The gp43 DNA polymerase of the RB69 bacteriophage (RB69 Pol) bears primary responsibility for the faithful and efficient replication of the viral genome. RB69 Pol belongs to the B-class of DNA polymerases and is closely related to T4 phage DNA polymerase. RB69 DNA Pol synthetizes DNA with high accuracy, introducing one mutation per 2 x 108 replicated bases. This high fidelity is achieved through the combined action of its polymerase (Pol) and 3′-5′-exonuclease (Exo) activities, which enable stringent selection of the correct incoming nucleotide and excision of the mismatches resulting from misincorporations.

Therefore, we took advantage of the Y567A substitution that has been shown to improve crystal quality without affecting the catalytic parameters of the enzyme (and references therein). We obtained crystals of a complex of the mutant polymerase, DNA and the dGpnpp non-hydrolyzable analog that diffracted to 2.30 Å resolution (ternary complex I). As expected, the ternary complex structure reveals an assembled active site with dGpnpp occupying the incoming dNTP binding pocket. Strikingly, however, while the base and sugar of the incoming nucleotide are found in positions that are consistent with other RB69 polymerase structures, both molecules in the ASU present an altered conformation for the three phosphate groups. As a consequence the α-phosphate is not properly aligned for catalysis. Furthermore, the D714A substitution drastically affects the metal coordination. Neither the dNTP binding metal, nor the catalytic metal ions are found in their expected positions. Interestingly, this aberrant active site conformation correlates with similar changes to those observed in the apo crystal structure, suggesting that the altered position of the incoming nucleotide is related to the conformation of D411 and, in turn, to the missing D714 side chain. As seen in the apo mutant structure, the D411 is flipped away from the active site and this correlates with the repositioning of the E686 and E716 side chains. Thus, the absence of the D714 side chain seems to cause the movement of the key metal-ligating D411 residue in the polymerase pocket and, as such, agrees with the observed decrease in the DNA polymerization rate.

>[2x]MKEFYLTVEQIGDSIFERYIDSNGRERTREVEYKPSLFAHCPESQATKYFDIYGKPCTRKLFANMRDASQWIKRMEDIGLEALGMDDFKLAYLSDTYNYEIKYDHTKIRVANFDIEVTSPDGFPEPSQAKHPIDAITHYDSIDDRFYVFDLLNSPYGNVEEWSIEIAAKLQEQGGDEVPSEIIDKIIYMPFDNEKELLMEYLNFWQQKTPVILTGWNVESFAIPYVYNRIKNIFGESTAKRLSPHRKTRVKVIENMYGSREIITLFGISVLDYIDLYKKFSFTNQPSYSLDYISEFELNVGKLKYDGPISKLRESNHQRYISYNIIAVYRVLQIDAKRQFINLSLDMGYYAKIQIQSVFSPIKTWDAIIFNSLKEQNKVIPQGRSHPVQPYPGAFVKEPIPNRYKYVMSFDLTSLYPSIIRQVNISPETIAGTFKVAPLHDYINAVAERPSDVYSCSPNGMMYYKDRDGVVPTEITKVFNQRKEHKGYMLAAQRNGEIIKEALHNPNLSVDEPLDVDYRFDFSDEIKEKIKKLSAKSLNEMLFRAQRTEVAGMTAQINRKLLINSLAGALGNVWFRYYDLRNATAITTFGQMALQWIERKVNEYLNEVCGTEGEAFVLYGDTDSIYVSADKIIDKVGESKFRDTNHWVDFLDKFARERMEPAIDRGFREMCEYMNNKQHLMFMDREAIAGPPLGSKGIGGFWTGKKRYALNVWAMEGTRYAEPKLKIMGLETQKSSTPKAVQKALKECIRRMLQEGEESLQEYFKEFEKEFRQLNYISIASVSSANNIAKYDVGGFPGPKCPFHIRGILTYNRAIKGNIDAPQVVEGEKVYVLPLREGNPFGDKCIAWPSGTEITDLIKDDVLHWMDYTVLLEKTFIKPLEGFTSAAKLDYEKKASLFDMFDF> DFINWL

Here, we identify an evolutionarily conserved hexapeptide sequence as the major aggregation-prone region (APR) of gastrointestinal peptides of the glucagon family: xFxxWL. We determine nine polymorphic crystal structures of the APR segments of glucagon-like peptides 1 and 2, and exendin and its derivatives. We propose that the pH-dependent changes of the protonation states of glutamate/aspartate residues of APRs initiate switching between the amyloid and the folded, monomeric forms of the hormones. Our results highlight the dual role of short aggregation core motifs in reversible amyloid formation and receptor binding.

Seven of the nine structures present an antiparallel (AP) backbone of class 7 or 8 topology, while 2 peptides, those of APRGLP2 and polymorph D of APRTc5b, form class 1 or class 4 steric zippers both comprising of parallel (PA) β-sheets. The glucagon-like APRs (APRGLP2 and APRGLP1) show an extensive contact surface (Sc = ~0.80; Area = ~160 Å2) along the extended, linear backbone of high complementarity, while exendin-like sequences (APRex-4 and APRTc5b) present generally smaller values (Sc = ~0.65; Area = ~110 Å2). Aromatic side chains form intrasheet aromatic ladders in the two parallel structures of APRGLP2 and APRTc5b (polymorph D), as well as in both polymorphic structures of APRex-4. Additionally, within a zipper, amide groups of Gln and Asn side chains can stabilize parallel β-sheets by axial H-bond ladders. The amyloid crystal structures of APRGLP1, APRGLP2, and APRex-4 revealed the nature of emerging interactions between charge-abolished side chains contributing to steric zipper stabilization.> EDRTLLADLARLGEWTGNGPRALGFWKQLLAGADDPALREHAWRLSLQMFDFDSAIEL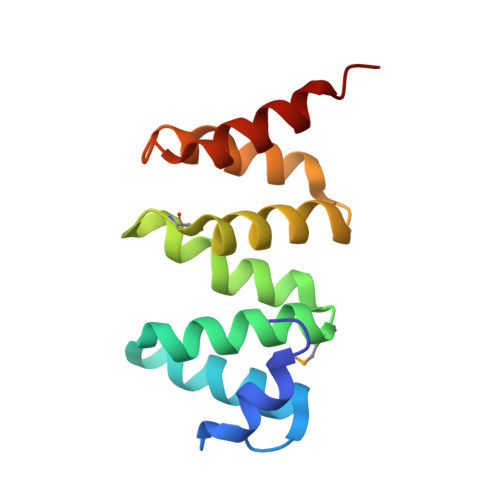LAPIGAQRQMTDEELDALVYSHETRGTPEEGEAWLRGYVQRYPKQRLAWQRLQQILEHTQ N-[3-(6-methyl-1H-indazol-3-yl)phenyl]prop-2-enamide | C17 H15 N3 O | 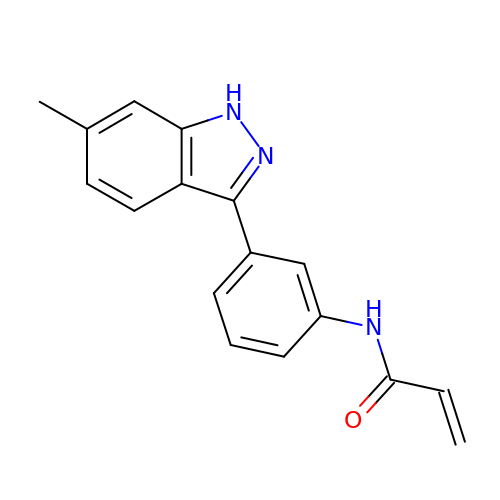YCMAZDUWLKXRRU-UHFFFAOYSA-N> WM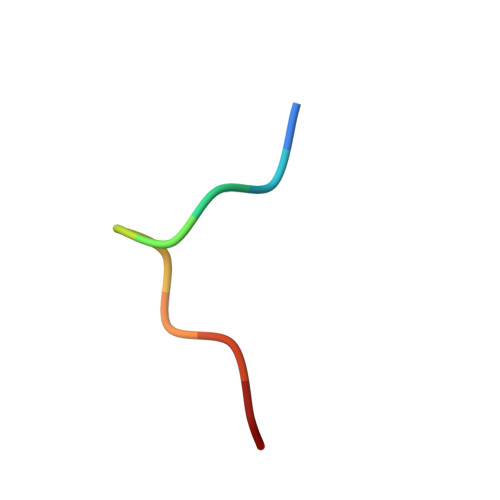DFDDDIPF> KVFERCELARTLKRLGMDGYRGISLANWMCLAKWESGYNTRATNYNAGDRSTDYG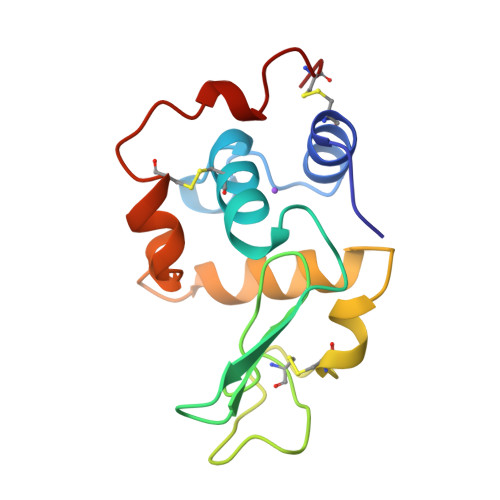IFQVNSRYWCNDGKTPGAVNAAHLSCSALLQDNIADAVAAAKRVVRDPQGIRAWVAWRNRCQNRDVRQYVQGCGV Quinolones act on type II topoisomerase–DNA complexes to prevent strand passage of the T-segment through the cleaved G-gate in the topoisomerase cycle. Quinolones trap the covalent enzyme–DNA cleavage complex, preventing DNA resealing and triggering cell death. The upper part of the topoisomerase complex consists of the E-subunit TOPRIM domain formed of four parallel β-sheets and surrounding α-helices. The WHD within the C-subunit together with the TOWER forms the U-groove-shaped protein region into which the G-gate DNA binds inducing a banana-shaped bend.

As part of our ongoing structural and biochemical studies aimed at new topoisomerase-targeting therapeutics, we have focused on topoisomerase IV–DNA complexes with ACHN-245 and ACHN-454, two novel 7,8-bridged fluoroquinolones developed and produced by Achaogen. However, they differ in having a heptacyclic ring system formed between the quinolone 8-position and the 2-position of the 3-aminopyrrolidin-1-yl substituent at position 7; this seven-membered ring contains a double bond in ACHN-245 and a cyclic ether in ACHN-454. Moreover, we report the structures of the topoisomerase IV–DNA cleavage complexes with ACHN-245 and ACHN-454 at 3.43 and 3.24 Å resolution, respectively. Within the S. pneumoniae topoisomerase IV complex, a 7,8-bridged quinolone is hemi-intercalated into each DNA strand and stacked against the DNA bases at the cleavage site (positions −1 and +1 of the 4 bp staggered cut in the 18mer DNA) as found now in many other Gram-negative and Gram-positive topoisomerase IV and gyrase complexes. The carboxyl at quinolone position 3, besides interacting with this magnesium ion, also makes interactions with ParC S79 and R117; the lengths of these interactions are similar for both drugs. The amino group on the 7-(3-aminopyrrolidin-1-yl) group makes key interactions with a cluster of two glutamates and an arginine (ParE E474, E475 and R456 in ParE) through a single oxygen of the carboxyl groups of the glutamates and the main chain carbonyl of R456. In both cases, the cyclopropyl group on N-1 of the quinolone is cocked out of the plane of the quinolone. The stacking interactions are very similar, but the cycloheptyl group of these Achaogen compounds projects towards R456 and D435 and if modified could form a scaffold for substituents which could span towards these and other residues and impart further contacts.

>[2x]MSNIQNMSLEDIMGERFGRYSKYIIQDRALPDIRDGLKPVQRRILYSMNKDSNTFDKSYRKSAKSVGNIMGNFHPHGDSSIYDAMVRMSQNWKNREILVEMHGNNGSMDGDPPAAMRYTEARLSEIAGYLLQDIEKKTVPFAWNFDDTEKEPTVLPAAFPNLLVNGSTGISAGYATDIPPHNLAEVIDAAVYMIDHPTAKIDKLMEFLPGPDFPTGAIIQGRDEIKKAYETGKGRVVVRSKTEIEKLKGGKEQIVITEIPYEINKANLVKKIDDVRVNNKVAGIAEVRDESDRDGLRIAIELKKDANTELVLNYLFKYTDLQINYNFNMVAIDNFTPRQVGIVPILSSYIAHRREVILARSRFDKEKAEKRLHIVEGLIRVISILDEVIALIRASENKADAKENLKVSYDFTEEQAEAIVTLQLYRLTNTDVVVLQEEEAELREKIAMLAAIIGDERTMYNLMKKELREVKKKFATPRLSSLEDTAKALEHHHHHH;>MGHHHHHHHHHHSSGHIDDDDKHMKNKKDKGLLSGKLTPAQSKNPAKNELYLVEGDSAGGSAKQGRDRKFQAILPLRGKVINTAKAKMADILKNEEINTMIYTIGAGVGADFSIEDANYDKIIIMTDADTDGAHIQTLLLTFFYRYMRPLVEAGHVYIALPPLYKMSKGKGKKEEVAYAWTDGELEELRKQFGKGATLQRYKGLGEMNADQLWETTMNPETRTLIRVTIEDLARAERRVNVLMGDKVEPRRKWIEDNVKFTLEEATVF[2x]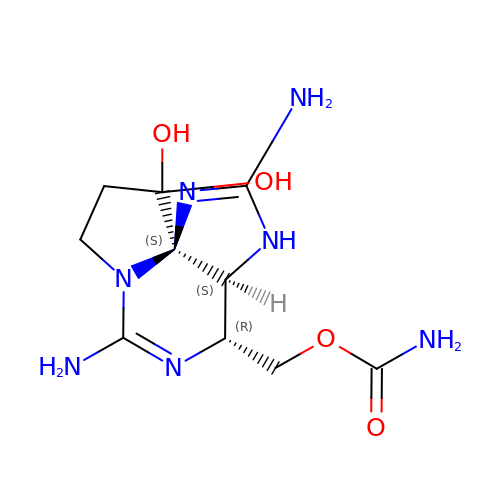[(3aS,4R,10aS)-2,6-diamino-10,10-dihydroxy-3a,4,9,10-tetrahydro-3H,8H-pyrrolo[1,2-c]purin-4-yl]methyl carbamate | C10 H17 N7 O4 | RPQXVSUAYFXFJA-HGRQIUPRSA-N> MKRLMLSAVLAAGVPAMPAMAEDWNDPQEPFAVFGSTYYVGVRGLSAVLIASPQGHILIDGGSPESAPQIAQHIRQLGFKLEDVKLILNSHEHFDHAGGISELQRLSGATVLASVQGEKVLRSGQPSKGDPQYGELPPMTPVANTRAVA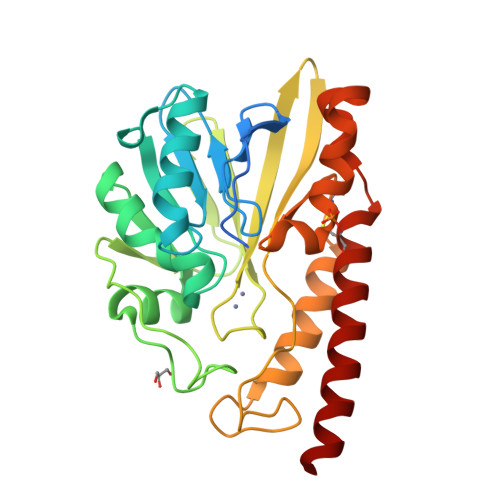DGEVVKLGPLAVTARYTPGHTQGGVSWTWRATENGKSAAMVYADSLNAFAAKPFRYSGSPAYPNALADIKKSIATVAALDCDILISAHPDAGDLWRRQARQAELGSAAFIDRQACRQYAERAGVRLQKKLAAEAAEK1-(2-HYDROXYETHYLOXYMETHYL)-6-PHENYL 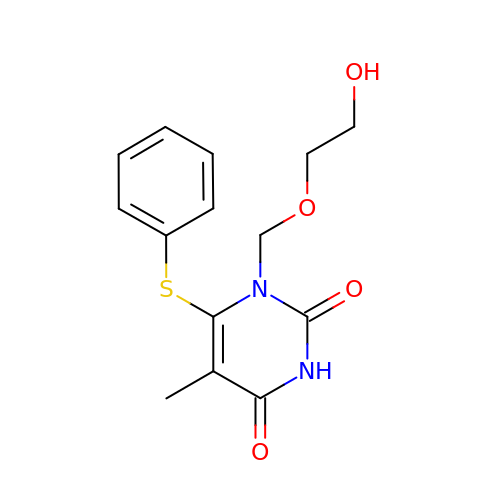THIOTHYMINE | C14 H16 N2 O4 S | HDMHBHNRWDNNCD-UHFFFAOYSA-N> GGGHMAKIIVKKSNPLKGSVKIDGAKNAVLPIIAATLLANGKSTLNGVPNLRDVHVISDLLRHVGAEVEYKENTLTVDASNIKTCEAPYELVRKMRASFLVMGPLLARFNSTKISMPGGCAIGTRPIDLHLKGFKALGAKIEMDHGFVEAATEKLVGNKLYLDFPSVGATENIMMAASLAEGTTIIENAAEEPEIVDLANFLNEMGADVKGAGTNTIKIKGVKELKGAEHNVIPDRIEAATYMVAAAMTKGDITVENVLMEHLKPVVAKLREAGCEITEMDNSVRVVGPKVLKPIDIKTLPHPGFPTDVQAQFMAMLTVANGTGVVIETVFENRFMHVAEFNRMGANIKIDGRSAVVNGVDELHGAAVNATDLRAGAALILCGLIAEGETQIGEIYHIQ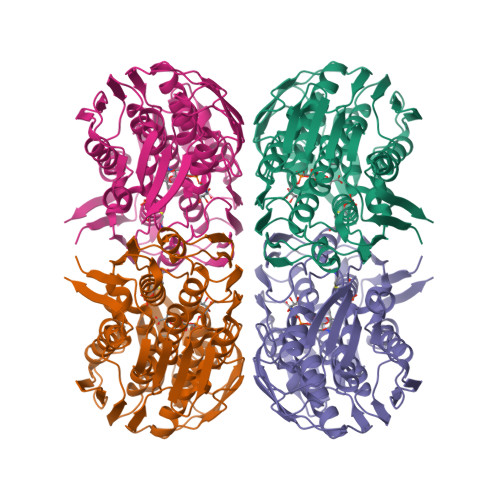RGYVDIDKKITALGGQIEIVED>[2x]MELRVGNRYRLGRKIGSGSFGDIY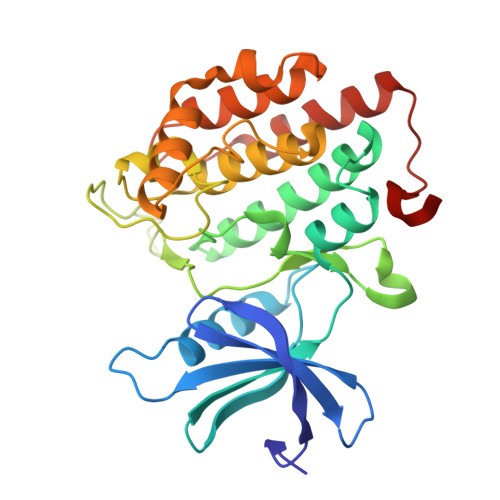LGTDIAAGEEVAIKLECVKTKHPQLHIESKIYKMMQGGVGIPTIRWCGAEGDYNVMVMELLGPSLEDLFNFCSRKFSLKTVLLLADQMISRIEYIHSKNFIHRDVKPDNFLMGLGKKGNLVYIIDFGLAKKYRDARTHQHIPYRENKNLTGTARYASINTHLGIEQSRRDDLESLGYVLMYFNLGSLPWQGLKAATKRQKYERISEKKMSTPIEVLCKGYPSEFATYLNFCRSLRFDDKPDYSYLRQLFRNLFHRQGFSYDYVFDWNMLK>[2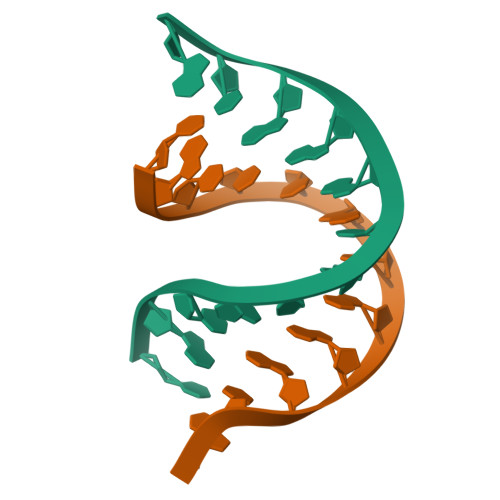x]CGCCCGCGGGCG>[2x]AARYDDILYFPASRYPETGAHISDAIKAGHSD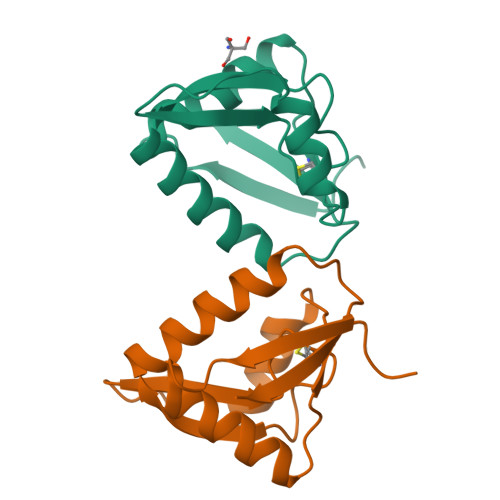VCTIERSGADKRRQESLKGIPTKPGFDRDEWPMAMCEEGGKGASVRYVSSSDNRGAGSWVGNRLSGFADGTRILFIVQ>[16x]EEIMRDDNMMFITKKMIEIRNLLQKVGQGSTVTLPSIVVIGSQSSGKSSVLEAIVGHEFLPKGSNMITRRPIELTLVNDPEAKVDYGEFPDLGLARVTDFSLIQKTLTELNQSVPESECVTDDPIRLTIHSPNIPDLSLIDLPGYIQVAGENQPRELKRKITELCDKYIRGPNIILAISAADTDLANSTALQASRRVDPRGERTIGVITKMDLVEPEKGAAILSDRQYPLKLGYVGVISKLPPQSGLFRRDTGNLLASINRNEKNYFGSHPTE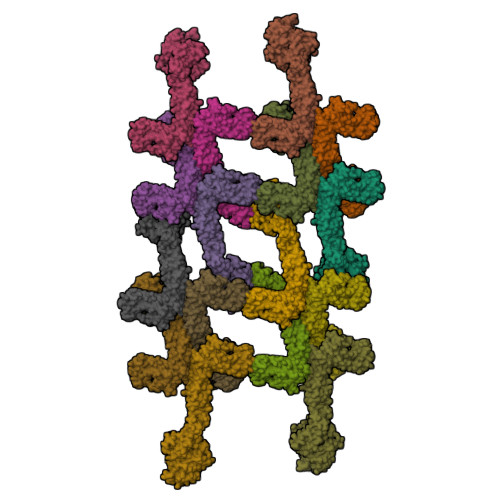FGPDSGVSTGVMTLRKKLLQVLEQQMSSKLNETTEAIQRELEETTYQFKVQYNEQPMSAESYLAASLDDFKHQFHEFASSFGRPQLQTLLKDALDQKVLDQLAARYWNRPIEDLSPAPREPDNIIDLPKADPDSPYWHRQLDTACSGLTRLGVGRLAATVAASAIQQHVEKLLDKSSFAKHPSARKVISDAAATVLADRSYATSDGIEISLKPYKFDPDIQPNEWAQGREHVVGVLQAELEQCQAAMKALENSVGGRKKLKEVMSFVDKARKGEIIVEGDHPSGAGGFSAALLARGREAVFLRDRADILSLRIQAAKSRQCKTLTNKYYCPEVFLDAVATKLAQTAVLFLNVEMLNDFYVRFPREVEAKLHEHMHAGGGLEKFAREDPKVRRHLDLIRRKELLETVLGKIEELHRISSGTAG>[2x]MESPSSEEEKPLAKMAFTLADRVTEEMLADKAALVVEVVEENYHDAPIVGIAVVNEHGRFFLRPETALADPQFVAWLGDETKKKSMFDSKRAAVALKWKGIELCGVSFDLLLAAYLLDPAQGVDDVAAAAKMKQYEAVRPDEAVYGKGAKRAVPDEPVLAEHLVRKAAAIWELERPFLDELRRNEQDRLLVELEQPLSSILAEMEFAGVKVDTKRLEQMGKELAEQLGTVEQRIYELAGQEFNINSPKQLGVILFEKLQLPVLKKTKTGYSTSADVLEKLAPYHEIVENILHYRQLGKLQSTYIEGLLKVVRPATKKVHTIFNQALTQTGRLSSTEPNLQNIPIRLE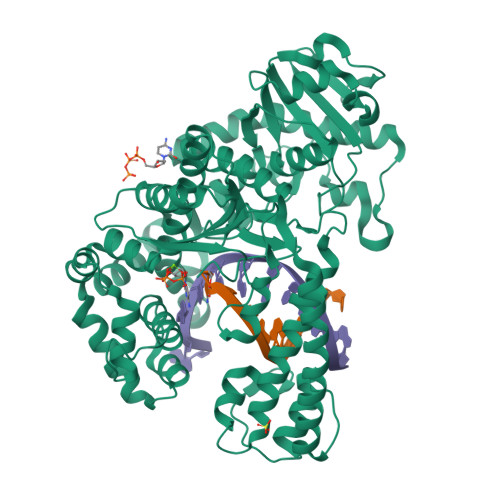EGRKIRQAFVPSESDWLIFAADYSQIELRVLAHIAEDDNLMEAFRRDLDIHTKTAMDIFQVSEDEVTPNMRRQAKAVNFGIVYGISDYGLAQNLNISRKEAAEFIERYFESFPGVKRYMENIVQEAKQKGYVTTLLHRRRYLPDITSRNFNVRSFAERMAMNTPIQGSAADIIKKAMIDLNARLKEERLQAHLLLQVHDELILEAPKEEMERLCRLVPEVMEQAVTLRVPLKVDYHYGSTWYDAK CA forms the capsid shell surrounding the viral core that protects and transports the viral genome and also interacts with host cell factors that are necessary for trafficking, nuclear entry and proviral integration. Further, we assemble particles from HML2 CArec in vitro and use single-particle cryogenic electron microscopy (cryo-EM) to determine the high-resolution structures of four different types of Fullerene shell assemblies. Our studies of HML2 CArec show that an ERV retains the ability to form capsid assemblies using the same architecture as exogenous viruses. Analysis of the shell structures reveals the intra- and inter-molecular interactions that drives CA assembly into pentamers and hexamers and their association into shells that encapsidate the retroviral genome.

The D5 particle is an elongated or capsular expansion of the T = 1 particle with polar regions identical to T = 1, but containing five equatorially inserted distorted hexamers, consistent with local two-fold (dihedral) symmetry. Moreover, adaptation of hexamers to the local environment is also a feature of our other D5 and D6 capsular assemblies, where hexamers interact with each other in the equatorial belt. Again, the pentamer conformation remains invariant and the hexamer six-fold symmetry is broken by NTD domain movements, changes in the NTD–CTD linker conformation and in the intra-hexamer CTD–NTD hydrogen bonding configuration and in the CTD radial position when interacting with either a neighbouring pentamer or hexamer. In the D5 and D6 particles, further configurations are possible depending on whether pentamers and hexamers are located at poles or are equatorial and interact either longitudinally or laterally. Nevertheless, all hexamer–pentamer interfaces still fall into group 2 and all hexamer–hexamer interfaces still fall into group 3, albeit in D6, the α8 displacement for the equatorial hexamer–hexamer interactions are larger than in D5, due to the lower curvature of the equatorial region. Exceptions were the N-terminal β-hairpin that contains a large loop insertion and is more mobile than in the crystal structure, and the NTD–CTD linker region of D5 and D6 equatorial hexamers that displayed weaker density.

>[9x]PVTLEPMPPGEGAQEGEPPTVEARYKSFSIKMLKDMKEGVKQYGPNSPYMRTLLDSIAHGHRLIPYDWEILAKSSLSPSQFLQFKTWWIDGVQEQVRRNRAANPPVNIDADQLLGIGQNWSTISQQALMQNEAIEQVRAICLRAWEKIQDPGSACPSFNTVRQGSKEPYPDFVARLQDVAQKSIADEKARKVIVELMAYENANPECQSAIKPLKGKVPAGSDVISEYVKACDGIGGAMHKAMLMAQLE>[2x]MTQDVTSGYSNLDLDLRDNGVCVVTLNRPDKRNALDVATIEELVTFFSTAHRKGVRAVVLTGAGDHFCAGLDLVEHWKADRSADDFMHVCLRWHE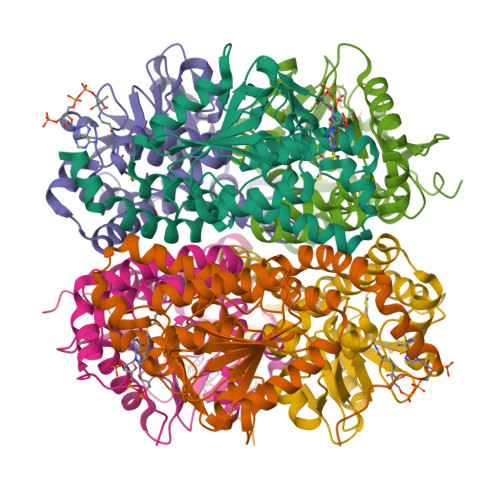AFNKMEYGGVPIIAALRGAVVGGGLALASAAHLRVMDQSTYFALPEGQRGIFTGGGATIRVSDMIGKYRMIDMILTGRVYQGQEAADLGLAQYITEGSSFDKAMELADKIASNLPLTNFAICSAISHMQNMSGLDAAYAEAFVGGIVNTQPAARERLEAFANKTAARVRPNSLEHHHHHH N-carboxy-L-cysteine | C4 H7 N O4 S | 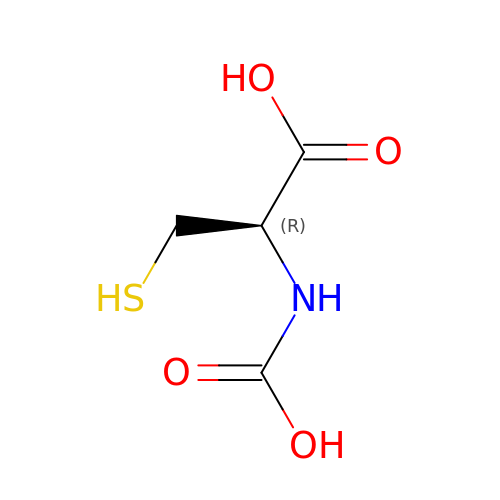ZJMMJMHTXLTBFW-REOHCLBHSA-N>GSGNQFPPIAAQDLPFVIKAGYLEKRRKDHSFLGFEWQKRWCALSKTVFYYYGSDKDKQQKGEFAIDGYDVRMNNTLRKDGKKDCCFEICAPDKRIYQFTAASPKDAEEWVQQLKFILQDLG[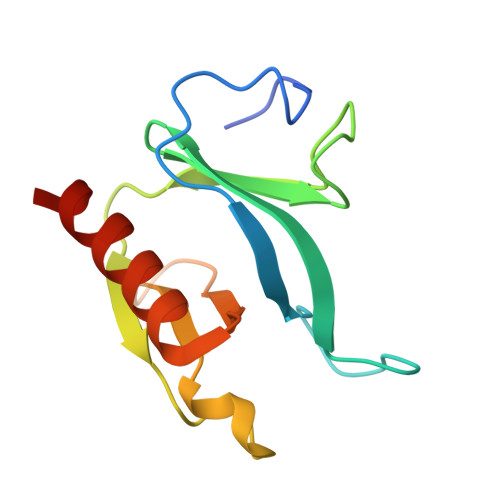4x]>MSEMTPREIVSELDQHIIGQADAKRAVAIALRNRWRRMQLQEPLRHEVTPKNILMIGPTGVGKTEIARRLAKLANAPFIKVEATKFTEVGYVGKEVDSIIRDLTDSAMKLVRQQEIAKNRARAEDVAEERILDALLPPAKNQWGEVENHDSHSSTRQAFRKKLREGQLDDKEIEIDVSAGVSMGVEIMAPPGMEEMTNQLQSLFQNLGSDKTKKRKMKIKDALKALIDDEAAKLINPEELKQKAIDAVEQNGIVFIDEIDKICKKGEYSGADVSREGVQRDLLPLVEGSTVSTKHGMVKTDHILFIASGAFQVARPSDLIPELQGRLPIRVELTALSAADFERILTEPHASLTEQYKALMATEGVNIAFTTDAVKKIAEAAFRVNEKTENIGARRLHTVMERLMDKISFSASDMNGQTVNIDAAYVADALGEVVENEDLSRFIL[12x];>[12x]TTIVSVRRNGQVVVGGDG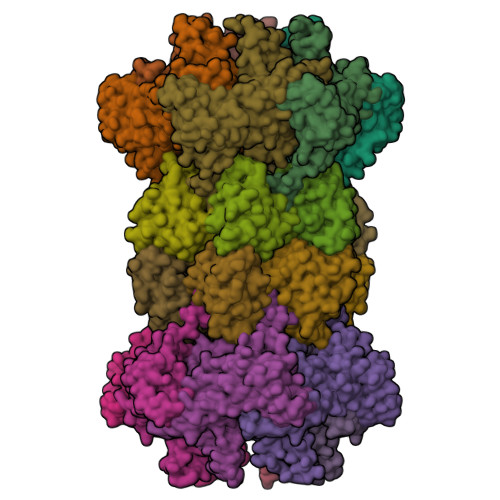QVSLGNTVMKGNARKVRRLYNGKVLAGFAGGTADAFTLFELFERKLEMHQGHLLKSAVELAKDWRTDRALRKLEAMLIVADEKESLIITGIGDVVQPEEDQILAIGSGGNYALSAARALVENTELSAHEIVEKSLRIAGDICVFTNTNFTIEELPN>MGSSHHHHHHSSGLVPAGSHSKVFIRSAINRVHQNSAANGGELPRIVFPEGTSTKVLKALATLVEEKICQPILLGYPERVKEKIKALDIPLLNDVSIVHPSSHPKYFSFVEKLYSLEQRKGINLGEAERLMADPNYFAAMMVNQGEADGMVSGSSINYADAVRPILQTIGVYKEGIPAGLNFVLLEDKFLVLADTTVNLNPTAEQCAQIALQAAKIVEYFGIEPRVAMLSYSNFSGAEGTPRKMKKAAEIARSLRPDLMIEGDMQADTAVNPEIMERLFPFSGLKGGANVLVFPNLESSNIAYKLIQQIGKAEVIGPFLTGVRRSANVLQRTTTVDGIVNSVVFTALEAQYIKEVLKSRGKK[6x]

Bacterial hybrid malic enzymes (MaeB grouping, multidomain) catalyse the transformation of malate to pyruvate, and are a major contributor to cellular reducing power and carbon flux. Distinct from other malic enzyme subtypes, the hybrid enzymes are regulated by acetyl-CoA, a molecular indicator of the metabolic state of the cell. The larger ME isoforms (hybrid enzymes) are predicted to be a fusion of two unrelated enzymes; a catalytic N-terminal ME subunit and a C-terminal phosphotransacetylase (PTA) domain. The PTA domain is homologous to PTA enzymes (that interconvert acetyl-CoA and phosphate to CoA and acetyl phosphate), yet they appear to lack critical catalytic residues and thus acts as a sensor instead.

An extension from d1 (residues 524–550, forming a loop with two helices that we term the 3′ loop) sits over the 3′-phosphate group, interacting via residues R535 and K538. Using HPLC as a readout, we were able to prevent acetyl-CoA binding by mutating R535 that makes a direct contact to the 3′ phosphate group. Variants R535E and R535A abolished acetyl-CoA binding, and generated an enzyme insensitive to allosteric inhibition by both CoA and acetyl-CoA, although these mutants retained ~70% activity to wild-type (wt) MaeB. We were also able to generate structures for R535E, R535A and N718D PTA domain variants, which demonstrate the same features as the wt PTAapo structure.>[2x]EFATMEAFEISDFKEHAKKKSMWAGALNKVTISGLMGVFTEDEDLMALPIHRDHCPALLKIFDEIIVNATDHERACHNKTKKVTYIKISFDKGVFSCENDGPGIPIAKHEQASLIAKRDVYVPEVASCHFLAGTNINKAKDCIKGGTNGVGLKLAMVHSQWAILTTADGAQKYVQHINQRLDIIEPPTITPSREMFTRIELMPVYQELGYAEPLSETEQADLSAWIYLRACQCAAYVGKGTTIYYNDKPCRTGSVMALAKMYTLLSAPNSTIHTATIKADAKPYSLHPLQVAAVVSPKFKKFEHVSVINGVNCVKGEHVTFLKKTINEMVVKKFQQTIKDKNRKTTLRDSCSNIFIVIVGSIPGIEWTGQRKDELSIAENVFKTHYSIPSSFLTSMTKSIVDILLQSISKKDNHKQVDVDKYTRARNAGGKRAQDCMLLAAEGDSALSLLRTGLTLGKSNPSGPSFDFCGMISLGGVIMN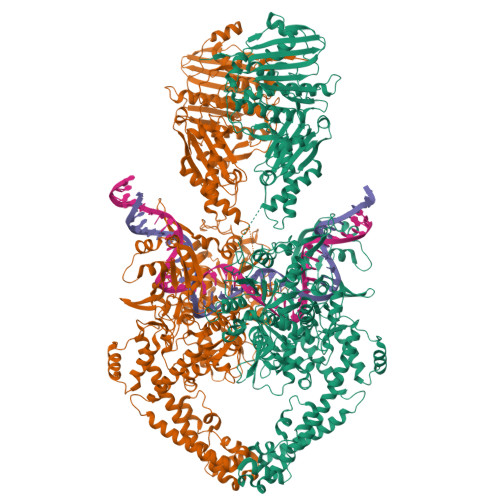ACKKVTNITTDSGETIMVRNEQLTNNKVLQGIVQVLGLDFNCHYKTQEERAKLRYGCIVACVDQDLDGCGKILGLLLAYFHLFWPQLIIHGFVKRLLTPLIRVYEKGKTMPVEFYYEQEFDAWAKKQTSLANHTVKYYKGLAAHDTHEVKSMFKHFDNMVYTFTLDDSAKELFHIYFGGESELRKRELCTGVVPLTETQTQSIHSVRRIPCSLHLQVDTKAYKLDAIERQIPNFLDGMTRARRKILAGGVKCFASNNRERKVFQFGGYVADHMFYHHGDMSLNTSIIKAAQYYPGSSHLYPVFIGIGSFGSRHLGGKDAGSPRYISVQLASEFIKTMFPAEDSWLLPYVFEDGQRAEPEYYVPVLPLAIMEYGANPSEGWKYTTWARQLEDILALVRAYVDKDNPKHELLHYAIKHKITILPLRPSNYNFKGHLKRFGQYYYSYGTYVISEQRNIITITELPLRVPTVAYIESIKKSSNRMTFIEEIIDYSSSETIEILVKLKPNSLNRIVEEFKETEEQDSIENFLRLRNCLHSHLNFVKPKGGIIEFNTYYEILYAWLPYRRELYQKRLMREHAVLKLRIIMETAIVRYINESAELNLSHYEDEKEASRILSEHGFPPLNHTLIISPEFASIEELNQKALQGCYTYILSLQARELLIAAKTRRVEKIKKMQARLDKVEQLLQESPFPGASVWLEEIDAVEKAIIKGRNTQWKFHENLYFQGHHHHHHHH> SKLLDNLRDTVRKFLTGSSSYDKAVEDFIKELQKSLISADVNVKLVFSLTNKIKERLKNEKPPTYIERREWFIKIVYDELSNLFGGDKEPKVIPDKIPYVIMLVGVQGTGKTTTAGKLAYFYKKKGFKVGLVGADVYRPAALEQLQQLGQQIGVPVYGEPGEKDVVGIAKRGVEKFLSEKMEIIIVDTAGRHGYGEEAALLEEMKNIYEAIKPDEVTLVIDASIGQKAYDLASKFNQASKIGTIIITKMDGTAKGGGALSAVAATG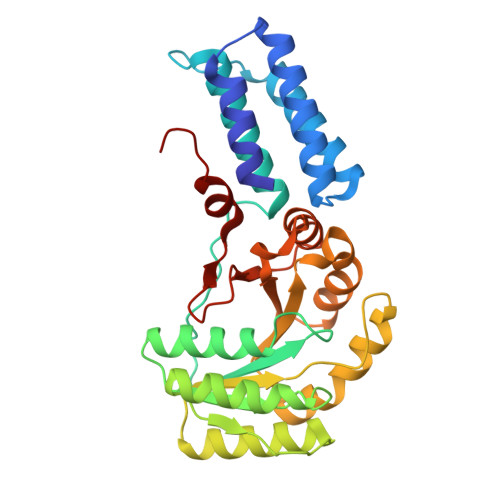ATIKFIGTGEKIDELEVFNPRRFVARLHHHH>GSFNSLEACLPATCLEPCVICQSRPKNGCIVHGRTGHLMACYTCAKKLKNRNKLCPVCREPIQSVVLTYMS[2x]

The importance of the ubiquitin ligase murine double mutant 2 (MDM2) as a key negative regulator of the tumour suppressor protein p53 has been studied extensively. Second, it promotes the proteasomal degradation of p53 by recruiting Ub conjugating enzyme (E2) thioesterified with ubiquitin (E2~Ub; ~ indicates thioester bond) via its RING domain and mediates ubiquitin (Ub) transfer from E2 to p53,8 where Ub is preferentially conjugated to lysine residues located in the C-terminal lysine rich region of p53.9 Although the relative importance of these mechanisms is context dependent, in vivo mouse studies with ligase defective MDM2 resulted in the same lethality as MDM2 knockout experiments. The RING domain of MDM2 has been discussed as an alternative target to stabilize p53.19 The rationale for this approach lies in MDM2′s ability to still bind and inhibit p53 when MDM2-mediated ubiquitination is abolished, thereby preventing uncontrolled activation of p53.8 The RING domain gains its E3 ligase activity through dimerization with either itself or the RING domain of its catalytic inactive homologue MDMX to form a homodimer or heterodimer, respectively. The dimeric RING domain arrangement is essential for E2~Ub binding and activation as demonstrated by co-crystal structures with UbcH5B–Ub (en dash indicates covalent complex).

We wondered whether the sequence dissimilarity induced structural differences that could account for the different aggregation tendencies of the MDM2 variants and performed protein crystallization for MDM2f and MDM2z. We obtained crystals for MDM2z and MDM2f, which diffracted to 2.87 and 2.27 Å, respectively. The unit cell for the MDM2z crystal contains two molecules of MDM2z, which form a dimer. The overall structure is similar to MDM2h (RMSD of 0.6 Å), where all secondary structure elements and the coordination of zinc ions are conserved. There was no electron density for the first 11 residues (407–417, corresponding to 423–433 in MDM2h), which are located N-terminal to the RING domain and partly involved in the formation of a 310-helix in MDM2h. A possible explanation for this observation could be the sequence difference for residues preceding the RING domain, which form a 310-helix in MDM2h but lack electron density in all MDM2f and MDM2z structures reported in this study. The helices are stabilized by a tight hydrophobic packing arrangement involving residues A434 and F490 of each protomer. In MDM2f and MDM2z, A434 is replaced with serine and cysteine, respectively. Both serine and cysteine would likely cause a steric clash and their polar side chains would disrupt the hydrophobic packing, thereby precluding a similar helical arrangement.3-{5-[(2E,4S)-2-imino-1,4-dimethyl-6-oxohexahydropyrimidin-4-yl]thiophen-3-yl}benzonitrile | C17 H16 N4 O S | 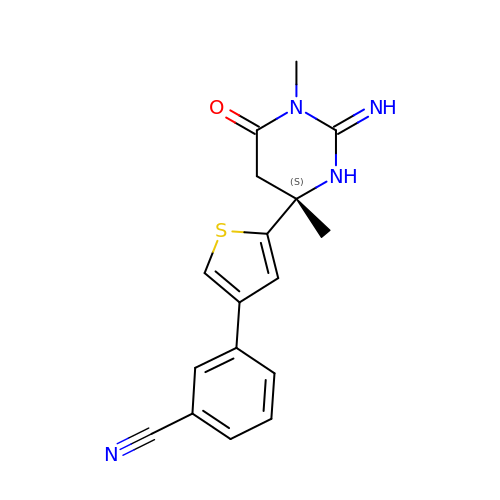MLNWGLXMDFUREO-KRWDZBQOSA-N>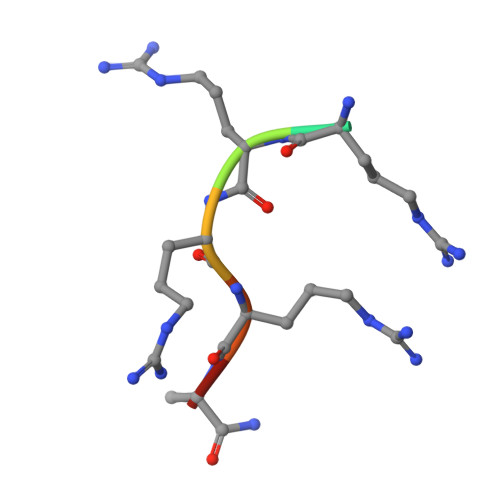 ARRRRAX> STGSKQRSQNRSKTPKNQEALRMANVAENSSSDQRQACKKHELYVSFRDLG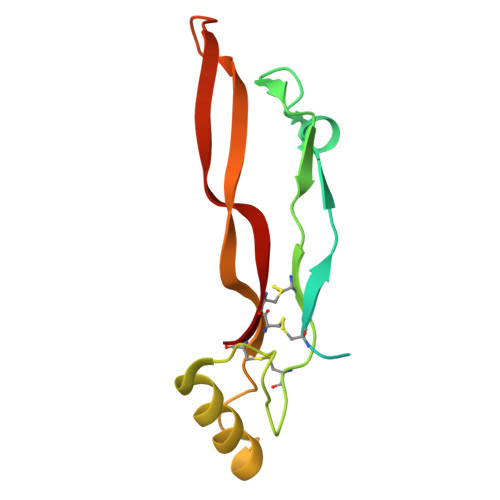WQDWIIAPEGYAAYYCEGECAFPLNSYMNATNHAIVQTLVHFINPETVPKPCCAPTQLNAISVLYFDDSSNVILKKYRNMVVRACGCH>GPGMSSLSNSLPLMEDVQGIRKAQKADGTATVMAIGTAHPPHIFPQDTYADVYFRATNSEHKVELKKKFDHICKKTMIGKRYFNYDEEFLKKYPNITSYDEPSLNDRQDICVPGVPALGTEAAVKAIEEWGRPKSEITHLVFCTSCGVDMPSADFQCAKLLGLHANVNKYCIYMQGCYAGGTVMRYAKDLAENNRGARVLVVCAELTIMMLRAPNETHLDNAIGISLFGDGAAALIIGSDPIIGVEKPMFEIVCTKQTVIPNTEDVIHLHLRETGMMFYLSKGSPMTISNNVEACLIDVFKSVGITPPEDWN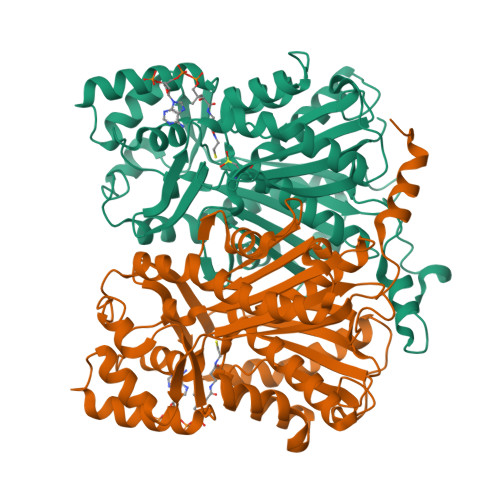SLFWIPHPGGRAILDQVEAKLKLRPEKFRAARTVLWDYGNMVSASVGYILDEMRRKSAAKGLETYGEGLEWGVLLGFGPGITVETILLHSLPLM[2x]>[2x]GPGSSRYDFFNVVTAICQLDKPHDYGYAIFTQLPDCTEIQFHLKNLPPGKHGCHIHKSGDRRNGCTSMGPHFNPFNGV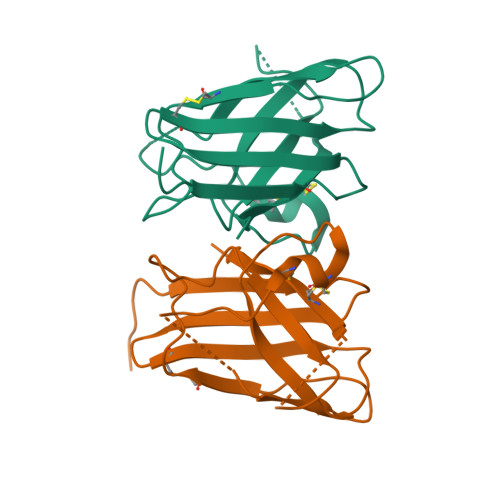HKDINIQHNHLGDLGNIVVNNNGECNEIICVKYLPLTGSNQIIGRGLVIHEKEDDLGMTNHPDSKTTGNSGDRIACGIIAYLN>[2x]GSHMNGHIYAVGGYDGSPDGHTHLNSVEAYDPERDEWSLVAPMNTRRSGVGVAVLDGHIYAVGGYDGHTHLNSVEAYDPERDEWHMVTPMNTRRSGVGVAVLNGHIYAVGGYDGSPDGHT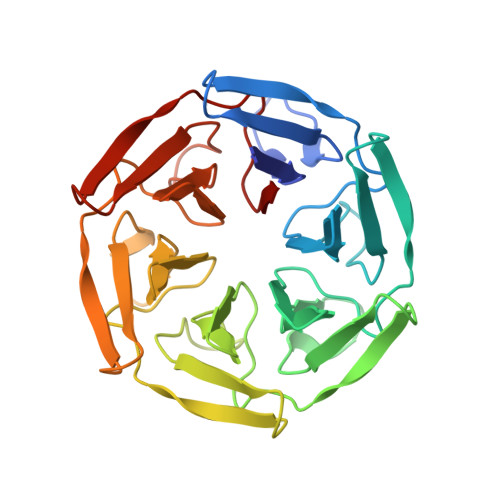HLNSVEAYDPERDEWSLVAPMNTRRSGVGVAVLDGHIYAVGGYDGHTHLNSVEAYDPERDEWHMVTPMNTRRSGVGVAVLNGHIYAVGGYDGSPDGHTHLNSVEAYDPERDEWSLVAPMNTRRSGVGVAVLDGHIYAVGGYDGHTHLNSVEAYDPERDEWHMVTPMNTRRSGVGVAVL>MNRDQEKIQIENEMNAMHGTIKEDILKDFEEFKGYLKKQVNRGKKLGLDDGKLVKSAAILGDYLAKHEEPQNGEEMLLQELWSVADEDEK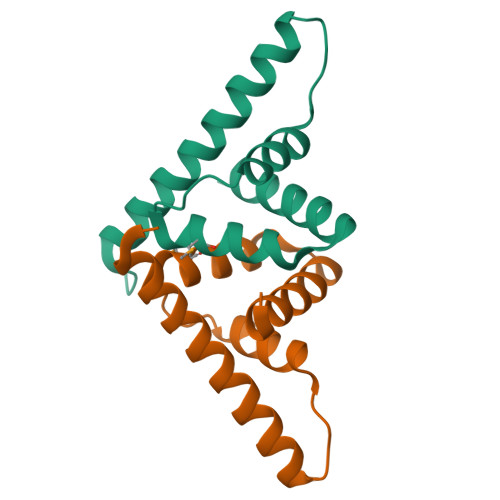EHLAQLLVKLVDKQ[4x]> GPDSMSDIKQLLKEAKQELTNRDYEETIEISEKVLKLDPDNYFAHIFLGKALSSLPASNNVSSNRNLERATNHYVSAAKLVPDNLLAWKGLFLLFRTTEVVPDILSYDEYFDLCGQYADALLKQEQSQVELINDIKLLKKTHPDCQKAFYQHLKPGSLMAETIGRHLSTPQDALLNLIKILSNIETTEIGKTLSQNRLKLKASDPDYQIKLNSFSWEIIKNSEIDQLYNQLVNILADDQKRSEIENQWLEYRIKVLKSMPLDVKKDFFTKVKEMVEDMVLVNHQSLLAWQKYFEWTDYEDLDNMDAPLIIKYFKKFPKDPLAMILYSWLSSKLSKYDIKSLESANKPPEGHKKTEKETDIKDVDETNEDEVKDRVEDEVKDRVEDEVKDQDEEAKEDEEEDLDDIEIGLLEEEVVTVLTENIVKCKNNILAHRILCQYYLLTKEYEAALPYIKNGISLIAYNIKDLGVHLPLTKREFSLDLATVYTYVDAPKDHNAALKLYDNILSGDFSNIQAKMGKGIIFIERKNWKDAMTLLTQVHEQSPNNLEVLSELSWSKAHMGYMDEALAGLDTVIKGIKGMDLRSIDFRALNLWRQAKVYIMKHASINDAKQ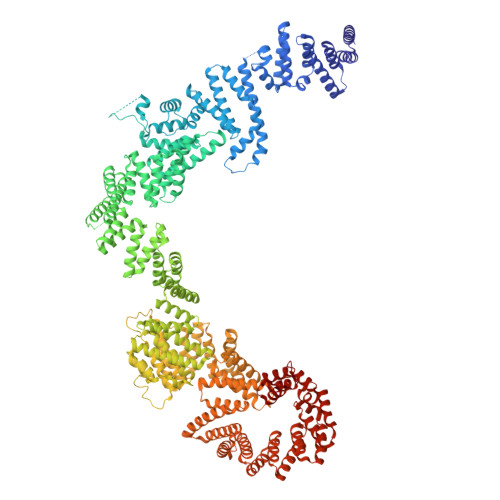ENVKCAFKLLIQSIKILDTFAPGFSTLGDIYCHYYKDHLRAFKCYFKAFDLDAGDYTAAKYITETYASKPNWQAASSIASRLIKGEKAKAELRSNNWPFRVVGIAHLEKQEESDSIEWFQSALRVDPNDVESWVGLGQAYHACGRIEASIKVFDKAIQLRPSHTFAQYFKAISLCDVGEYLESLDILEKVCQEAATEESFQIGLVEVLMRCSLDLYSQGFLLKSVSIAKDTIERIKIIISELKCENQQVWIYLSQVLRLFIWIESKVDTLPVESLVSIFENSQFSGSEEIDSVDNIKIDTLLDSTTDDNVSIACKFLILASKYSVSDQKFTDIAGTVRASYWYNIGISELTAFITLKEPQYRDAAIFAFKKSIQLQSNTSETWIGLGIATMDINFRVSQHCFIKATALEPKATNTWFNLAMLGLKKKDTEFAQQVLNKLQSLAPQDSSPWLGMALILEEQGDIIGSSKLFAHSFILSNGRSKAAQFMYAKNVLENHINNGDDERDIETVEKLTTASIALEQFFKKSPDSQFALQCALLTLERLHHYENANELANRLIGILEKKFEKTQDERELFNFAIIKGQFARIHLGLGNFELSIENADLSQGIISESSDEKSMKTKISNHICLGLSYFFLNDFDQTLNQFQELLSISKDSKHLVVLIAKVLYDVGESDTKEIALQELTEYIATSGADLLVTLTIAAMSILDDKREDLSIILEELKALPLSKQIIDKHKDAPYLIEEITKRLYRNDTGKQVWQRSAYFFPNNLKVWERLDKNIQRRIASNGQNKVTAEEMSKLYCESKNLRSIQRGMFLCPWNVTAVKALNECF> MESVAAESAPAPENEHSQETPESNSSVYTTFMKSHRCYDLIPTSSKLVVFDTSLQVKKAFFALVTNGVRAAPLWDSKKQSFVGMLTITDFINILHRYYKSALVQIYELEEHKIETWREVYLQDSFKPLVCISPNASLFDAVSSLIRNKIHRLPVIDPESGNTLYILTHKRILKFLKLFITEFPKPEFMSKSLEELQIGTYANIAMVRTTTPVYVALGIFVQHRVSALPVVDEKGRVVDIYSKFDVINLAAEKTYNNLDVSVTKALQHRSHYFEGVLKCYLHETLEAIINRLVEAEVHRLVVVDEHDVVKGIVSLSDILQALVLTGGEK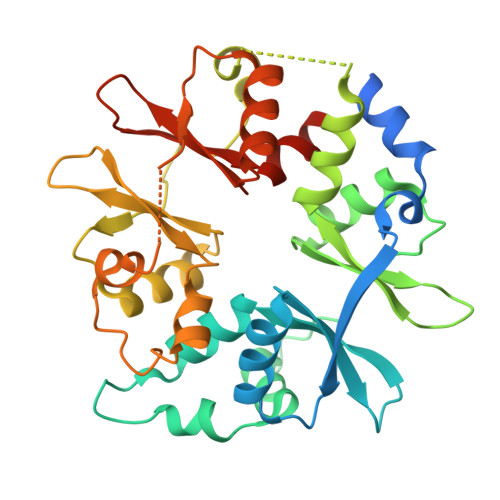KP>[20x]GAMGSGIQPNVNEYMFSNKFKARVMVSRKAPEGVTVNDTYDHKEDILKYEWFEFILPEGNFSATMTIDLMNNAIIDNYLEIGRQNGVLESDIGVKFDTRNFRLGWDPETKLIMPGVYTYEAFHPDIVLLPGCGVDFTESRLS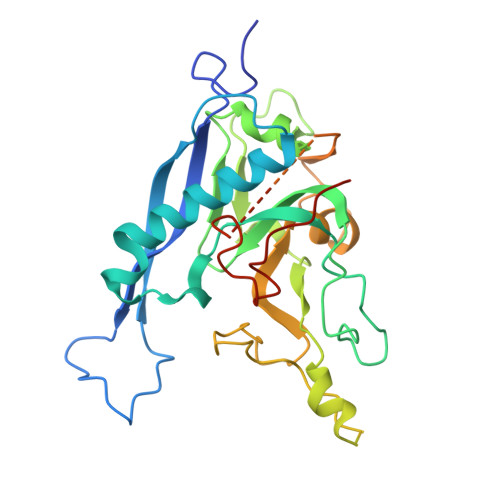NLLGIRKRHPFQEGFKIMYEDLEGGNIPALLDVTAYEESKKDTTTETTTKKELKIQPLEKDSKSRSYNVLEDKINTAYRSWYLSYNYGNPEKGIRSWTLLTTSDVTCGANGDSGNPVFSKSFYNEQAVYSQQLRQATSLTHVFNRFPENQILIRPPAPTITTVSENVP Human herpesvirus 6B (HHV-6B), a β-herpesvirus that significantly threatens immunocompromised individuals, currently lacks targeted antiviral therapies or vaccines. For HHV-6B, entry into susceptible cells—such as T cells, neurons, and salivary gland cells—is mediated by the fusion protein gB and the heterotetrametric gH/gL/gQ1/gQ2 complex. Through a structural transition from a prefusion to a postfusion conformation, gB mediates viral and host membranes fusion, a critical step conserved across herpesviruses. As gB not only mediates the essential membrane fusion step but also affects cellular tropism, it represents a promising target for blocking viral infection.

In this study, we determined the cryo-electron microscopy (cryo-EM) structure of the HHV-6B gB ectodomain in the postfusion conformation at 2.8 Å resolution. Specifically, the two fusion loops of HHV-6B gB, 102VGVV105 and 187WLY189, were replaced with 102HRTT105 and 187ATH189, respectively, in the final plasmid construct. Like other herpesvirus gB, HHV-6B gB forms a typical trimer with three protomers tightly packed together, resembling a long, rod-like structure. The ectodomain of each HHV-6B gB protomer is divided into five distinct structural domains. Each protomer contains five intrachain disulfide bonds, with no interchain disulfide bonds present in the trimer. The DIII long α-helix of each protomer together establishes a central coiled coil of the trimeric gB, and at its apex, DIII folds back nearly 180°, which contributes to a six-helix arrangement at the apex. In our resolved structure, the HHV-6B gB N-terminus, starting shortly after the predicted signal peptide (residues 1–19), directly forms a short β-strand with residues 27YIR29 that contributes to the formation of DIV. In HHV-6B, the first β-strand is positioned on the outer edge of the DIV and interacts with the central region of DIV to create an antiparallel β-sheet. For our HHV-6B gB construct, which did not include mutations to prevent furin cleavage, we observed a relatively low proportion of cleaved protein, and the structure we resolved corresponds to the intact furin site. Our structural analysis of the HHV-6B gB 396RRRR|D400 furin site is consistent with previous hypotheses, showing that it is an exposed loop on the exterior of the gB trimer that does not interact with the main gB body.

>[3x]MSKMRVLFLAVFLMNSVLMIYCDSDDYIRAGYNHKYPFRICSIAKGTDLMRFDRDISCSPYKSNAKMSEGFFIIYKTNIETYTFPVRTYKNELTFPTSYRDHRTTYFLDRTVMGLAMPVYEANLVNSRAQCYSAVAIKRPDGTVFSAYHEDNNKNETLELFPLNFKSVTNKRFITTKEPYFARGPLATHSTSTSLNCIVTEATAKAKYPFSYFALTTGEIVEGSPFFDGSNGKHFAEPLEKLTILENYTMIEDLMNGMNGATTLVRKIAFLEKGDTLFSWEIKEENESVCMLKHWTTVTHGLRAETDETYHFISKELTAAFVASKESLNLTDPKQTCIKNEFEKIITDVYMSDYNDAYSMNGSYQIFKTTGDLILIWQPLVQKSLMVLEQGSVNLRRRRDLVDVKSRHDILYVQLQYLYDTLKDYINDALGNLAESWCLDQKRTITMLHELSKISPSSIVSEVYGRPISAQLHGDVLAISKCIEVNQSSVQLYKSMRVVDAKGVRSETMCYNRPLVTFSFVNSTPEVVLGQLGLDNEILLGDHRTEECEIPSTKIFLSGNHAHVYTDYTHTNSTPIEDIEVLDAFIRLKIDPLENADFKLLDLYSPDELSRANVFDLENILREYNSYKSALYT>[4x]MHHHHHHGSENLYFQGSMPEESSPRRTPQSIPYQDLPHLVNADGQYLFCRYWAPTGTPKALIFVSHGAGE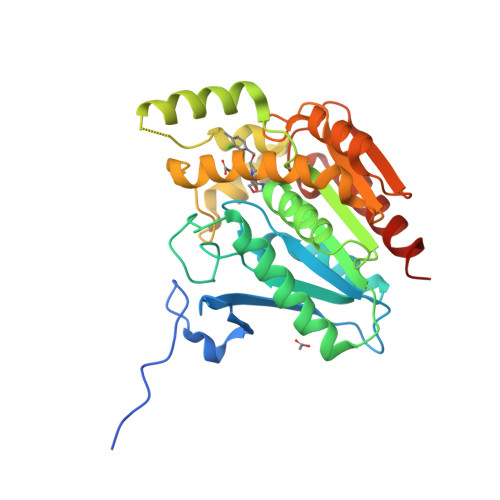HSGRYEELARMLMGLDLLVFAHDHVGHGQSEGERMVVSDFHVFVRDVLQHVDSMQKDYPGLPVFLLGHSMGGAIAILTAAERPGHFAGMVLISPLVLANPESATTFKVLAAKVLNSVLPNLSSGPIDSSVLSRNKTEVDIYNSDPLICRAGLKVCFGIQLLNAVSRVERALPKLTVPFLLLQGSADRLCDSKGAYLLMELAKSQDKTLKIYEGAYHVLHKELPEVTNSVFHEINMWVSQRTATAGTASPP>[2x]MELWLVRHGETLWNREGRLLGWTDLPLTAEGEAQARRLKGALPSLPAFSSDLLRARRTAELAGFSPRLYPELREIHFGALEGALWETLDPRYKEALLRFQGFHPPGGESLSAFQE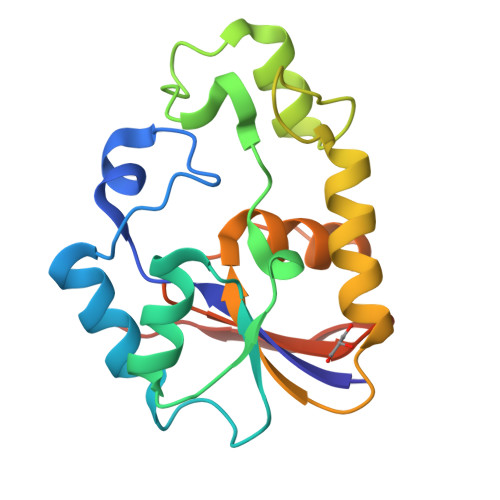RVFRFMEGLKAPAVLFTHGGVVRAVLRALGEDGLVPPGSAVAVDWPRRVLVRLALDGEEATG>MELTDEEASFLTRRQLLALSENGDLPDDIEYEVDLDLKFANNRLKRAYIALQAWKKAFYSDPFNTAANWVGPDVCSYKGVFCAPALDDPSVLVVAGIDLNHADIAGYLPPELGLLTDVALFHVNSNRFCGVIPKSLSKLTLMYEFDVSNNRFVGPFPTVALSWPSLKFLDIRYNDFEGKLPPEIFDKDLDAIFLNNNRFESTIPETIGKSTASVVTFAHNKFSGCIPKTIGQMKNLNEIVFIGNNLSGCLPNEIGSLNNVTVFDASSNGFVGSLPSTLSGLANVEQMDFSYNKFTGFVTDNICKLPKLSNFTFSYNFFNGEAQSCVPGSSQEKQFDDTSNCLQNRPNQKSAKECLPVVSR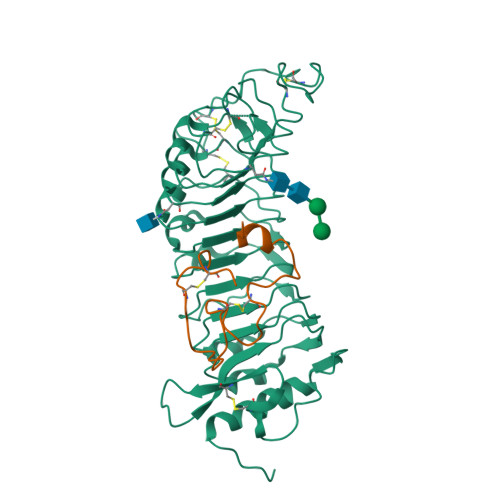PVDCSKDKCAGGLEGSENL[5x];>MGRRQLARGRRYIGYDALKKNNVPCSRRGRSYYDCKKRRRNNPYRRGCSAITHCYR[5x]Ene-reductases (ERs), NAD(P)H-dependent flavoproteins from the old yellow enzyme (OYEs) family, are powerful biocatalysts for the asymmetric reduction of activated alkenes, generating the products up to two new stereogenic centers with excellent enantioselectivities. To expand the OYEs toolbox, a new thermophilic-like OYE (AfOYE1) was identified from Aspergillus flavus strain NRRL3357. The sequence alignments showed that AfOYE1 conserved the two fingerprint motifs of the thermophilic-like OYE homologs and the catalytic residues of OYEs, including His211, His214, and Tyr216. AfOYE1 could accept cyclic enones, acrylamide, nitroalkenes, and α, β-unsaturated aldehydes as substrates and had excellent enantioselectivity toward prochiral alkenes (> 99% ee).

The UV–VIS absorption spectra of the purified AfOYE1, released flavin, and standard FMN suggested that AfOYE1 contained an FMN molecule as its prosthetic group and the FMN was non-covalently bound to the protein. The further crystal structure of AfOYE1 revealed that the “cap” region from Ala132 to Thr182, the loop of Ser316 to Gly325, α short helix of Arg371 to Gln375, and the C-terminal “finger” structure endow the catalytic cavity of AfOYE1 quite deep and narrow, and flavin mononucleotide (FMN) heavily buried at the bottom of the active site tunnel. As shown by the difference electron density map Fo-Fc, the si-face of the FMN faced the solvent, while the re-side was in contact with the protein backbone tightly via the extensive hydrogen bonding and hydrophobic interactions with the side chain and main chain elements. Meanwhile, the histidine pair (His211/His214) together with the highly conserved proton donor Tyr216 interacts with a buffer-sourced chloride anion and is positioned on the si-face of the isoalloxazine ring of FMN. It indicated that His/His together with Tyr 216 participated in the binding and correct orientation of substrate. The superposition structures of AfOYE1 with BfOYE4 and AnOYE8, with an r.m.s.d. of 0.694 Å and 0.588 Å, respectively, showed that they have similar monomer folding, except the α6-helix for the residues (from Phe271 to Glu280), the loop region (from Ser316 to Gly325), and the cap subdomain region (from Ala132 to Thr182). The protruding α6-helix and the long N-terminal loops of AfOYE1 work dimerization function in multi-asymmetry units. The loop region from Ser316 to Gly325 runs on the enzyme surface and reaches the active site entrance, which contributes to the size and feature of the catalytic cavity. The C-terminal α helix of each monomer (from Thr395 to Phe401) points to the active sites of the adjacent monomer, and the “finger” residue Trp399 interacts with the respective FMN flavin group at a distance of 3.8 Å. The novel structure of the loop of Ser316 to Gly325 narrows the entrance of the catalytic pocket.

>[2x]GISYYTPAQVPPAGTQVEGSTKLFSPLTIRGVTFPNRLFLAPLCQYSAKDGYANDWHLTHIGGIVQRGPGLAIMEATAVQKVGRITPQDLGLYDDGHIEPLKRITEFAHSQSQKIGIQLAHAGRKASAVAPWLSGNAMAVKEVGGWPDDIVAPSAIPQEEGINAVPKVLTGEDIGVLKKDWAEAAKRAVRANFDAIEIHAAHGYLLHQFLSPVSNRRTDKYGGSFENRVRILLEICEEVRAVIPTAMPLLVRISATDWFEFDDNLTKEFPESWTVAQSIRLALLLADRGVDLVDVSSGGIHAKSAIAIRSGPGYQVHFAQEIKKAVGEKLLISAVGGIKTGALAEEVVQSGIDAVQAGRWFQQNPGLVRAFANELGVKVRMATQIDWSFE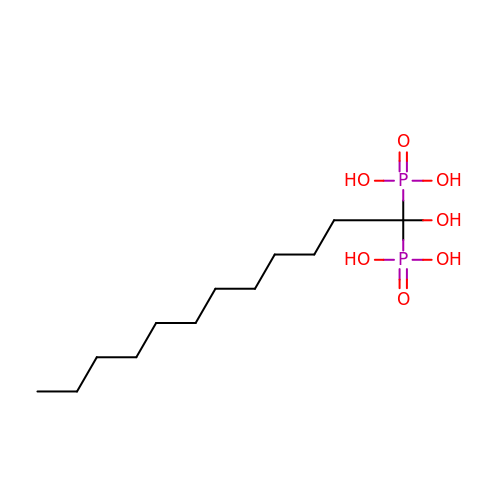(1-HYDROXYDODECANE-1,1-DIYL)BIS(PHOSPHONIC ACID) | C12 H28 O7 P2 | KKVZONPEMODBBG-UHFFFAOYSA-N Toscana virus is an enveloped negative-strand ribonucleic acid (RNA) virus that belongs to the genus phlebovirus in the Bunyaviridae family. The genome of phleboviruses, like other bunyaviruses, is tightly packed with N into ribonucleoprotein complexes (RNPs). In this study, we have elucidated structures of the hexameric RNA-free (apo) N and of hexameric N in complex with a single-stranded nonameric RNA. As in the RVFV N structure, each N monomer consisted of a core domain comprised of two α-helical lobes (the upper and the lower lobe), and an amino-terminal α-helical arm which was divided by a short linker, hinge II, in α1 and α2.

The RNA-containing N crystals had 24 N and 12 RNA molecules in the asymmetric unit, which were arranged in four almost identical hexameric rings. In agreement with our ITC data, only every second N bound an RNA molecule, whereas the central RNA-binding cleft of the neighboring monomer was empty. In all 12 RNA-bound Ns of the asymmetric unit, the 9-mer RNA occupied a defined position in a positively charged cleft at the inside of the hexameric ring, where the first and the last residue of the RNA could clearly be distinguished in the electron density. Tyr32 stacks against the base of G2, while Tyr32 of the neighboring subunit stacks against the base of uridine 9 (U9). In this way, each second N sequesters seven ribonucleotides, while two overlapping nucleotides are bound by neighboring subunits. However, the amino-terminal arm of the RNA-bound subunits is considerably displaced against the N core domain when compared to the apo structure or the RNA-free Ns in the RNP. Every second N monomer was laterally displaced relative to the neighboring N leading to a staggered assembly of the hexameric ring. In this way, the six-fold symmetry in the N hexamer was broken, resulting in three-fold symmetry of the RNP. However, the simultaneous binding of Lys204 and Lys79 of the adjacent subunit to the phosphate backbone of the RNA led to a 45° rotation between the subunits, with Tyr32 working as a pivot point. This domain movement created a new inter-subunit interface of 480 Å2 at the outside of the hexamer, which did not involve the amino-terminal arm.

>[21x]MSDENYRDIALAFLDESADSGTINAWVNEFAYQGFDPKRIVQLVKERGTAKGRDWKKDVKMMIVLNLVRGNKPEAMMKKMSEKGASIVANLISVYQLKEGNPGRDTITLSRVSAAFVPWTVQALRVLSESLPVSGTTMDAIAGVTYPRAMMHPSFAGIIDLDLPNGAGATIADAHGLFMIEFSKTINPSLRTKQANEVAATFEKPNMAAMSGRFFTREDKKKLLIAVGIIDEDLVLASAVVRSAEKYRAKVGK;>MSDENYRDIALAFLDESADSGTINAWVNEFAYQGFDPKRIVQLVKERGTAKGKDWKKDVKMMIVLNLVRGNKPEAMMKKMSEKGASIVANLISVYQLKEGNPGRDTITLSRVSAAFVPWTVQALRVLSESLPVSGTTMDAIAGVTYPRAMMHPSFAGIIDLDLPNGAGATIADAHGLFMIEFSKTINPSLRTKQANEVAATFEKPNMAAMSGRFFTREDKKKLLIAVGIIDEDLVLASAVVRSAEKYRAKVGK[2x];> MSDENYRDIALAFLDESADSGTINAWVNEFAYEGFDPKRIVQLVKERGTAKGRDWKKDVKMMIVLNLVRGNKPEAMMKKMSEKGASIVANLISVYQLKEGNPGRDTITLSRVSAAFVPWTVQALRVLSESLPVSGTTMDAIAGVTYPRAMMHPSFAGIIDLDLPNGAGATIADAHGLFMIEFSKTINPSLRTKQANEVAATFEKPNMAAMSGRFFTREDKKKLLIAVGIIDEDLVLASAVVRSAEKYRAKVGK>[2x]GSAMGSSAADQQFYGQLQQELPQMVQQINSSDMQEQLAATVKFRQILSREHNPPIDIVIQSGVVPTLVNFMNENQPEMLQLEAAWALTNIASGTSAQTQVVVDAGAVPLFIQLLYTGSVELQEQAIWALGNVAGDSTSYRDYVLQCSAMEPILSLFNSEKVTLIRTATWTLSNLCR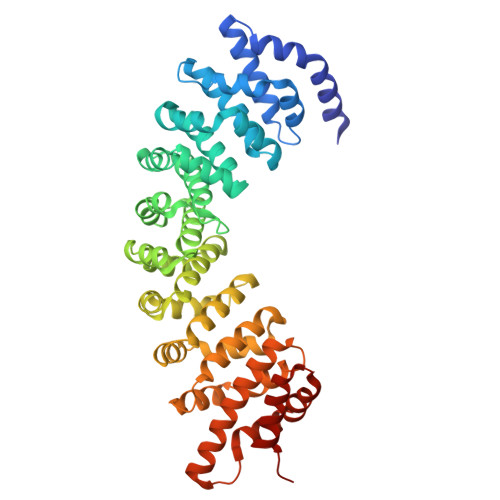GKKPQPDWSIVSKALPTLAKLIYSFDNETLIDACWAISYLSDGPAEAIQAVIDARIPKRLVELLSHQSTLVQTPALRAVGNIVTGNDLHTQVVINCGVLSALRNLLSSPKESIRKEACWTISNITAGNTEQIQAVVDANLIPPLIKLLETAEYKIKKEACWAISNASSGGLQRPEIIRYMVSQGCIKPLCDLLEIADNRIIEVTLDALENILKMGETDKEARGLAINENADLIEKAGGMEKIFNCQQNENDRIYEKAYKIIETYFGEEDDT>[12x]MKKILLLNGPNLNMLGKREPHIYGSQ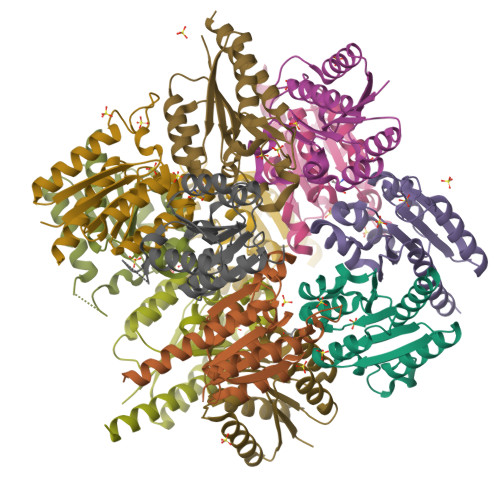TLSDIEQHLQQSAQAQGYELDYFQANGEESLINRIHQAFQNTDFIIINPGAFTHTSVAIRDALLAVSIPFIEVHLSNVHAREPFRHHSYLSDVAKGVICGLGAKGYDYALDFAISELQKIQLGEMMNG In metazoans, the α/β heterodimeric hypoxia-inducible factor (HIF) complex activates the expression of hundreds of target genes in response to hypoxia, including those involved in cell growth, apoptosis, energy metabolism and angiogenesis. The activities of both the PHDs and FIH are suppressed by limiting oxygen, resulting in HIFα stabilization and activation of the HIF system. Most of these compounds likely bind to the active site iron and compete with 2-oxoglutarate (2OG). Many bind in the pocket occupied by the 2OG (CH2)2COOH side chain, and as a consequence contain a carboxylic acid, which is often undesirable from a pharmacological perspective.

Recently, a set of tricyclic PHD inhibitor with linked pyridine-carboxylate, dihydropyrazole and triazole rings, such as 1 and IOX4 has been reported with one compound being in clinical development. This series has the potential for more than one mode of iron chelation and 2OG competition; we were particularly interested in the possibility that the triazole (an established carboxylate mimic), rather than the pyridine-carboxylate (an established 2OG mimic) might occupy the 2OG (CH2)2COOH binding pocket. To test this proposal, we prepared and studied both the acid and tertiary butyl ester (IOX4) of the ‘tricyclic series’, both reported as PHD inhibitors, but of uncharacterized selectivity and mechanism of action. Using an antibody-based (AlphaScreen) in vitro hydroxylation assay for PHD2 catalysis, both 1 and IOX4 were found to potently inhibit PHD2 with IC50 values of 4.8 nM and 1.6 nM, respectively. To obtain insights into the mode of PHD inhibition by the dihydropyrazoles, we made attempts to crystallize the PHD2 catalytic domain (residues 181–426) in complex with 1 or IOX4; a crystal structure of PHD2.Mn(II).1 was obtained. In the PHD2.Mn(II).1 complex, the inhibitor coordinates to Mn(II) in a bidentate manner via the nitrogen atoms of its pyridine and pyrazolone rings. In contrast to previously observed binding mode for other PHD inhibitors occupying the 2OG binding site such as IOX3, 2 and NOG, the pyridine-based chain of 1 extends towards the entrance of the active site and is positioned to make electrostatic interactions with Arg-322 (which is known to be involved in substrate binding). The 2OG C-5 carboxylate binding site of PHD2 which is reported to bind a ligand carboxylate in other PHD2.inhibitor complex structures,is occupied by the triazole ring of 1. Based on modelling studies, IOX4, for which we have not obtained a crystal structure, is predicted to bind in an analogous manner to 1, with its tert-butyl group protruding towards the entrance of the active site.

>[3x]GSHMASPNGQTKPLPALKLALEYIVPCMNKHGICVVDDFLGKETGQQIGDEVRALHDTGKFTDGQLVSQKSDSSKDIRGDKITWIEGKEPGCETIGLLMSSMDDLIRHCNGKLGSYKINGRTKAMVACYPGNGTGYVRHVDNPNGDGRCVTCIYYLNKDWDAKVSGGILRIFPEGKAQFADIEPKFDRLLFFWSDRRNPHEVQPAYATRYAITVWYFDADERARAKVKYLTGEKGVRVELNKPSDSVGKDVF[({5-[4-(cyclopropyloxy)phenyl]pyridin-3-yl}amino)methanediyl]bis(phosphonic 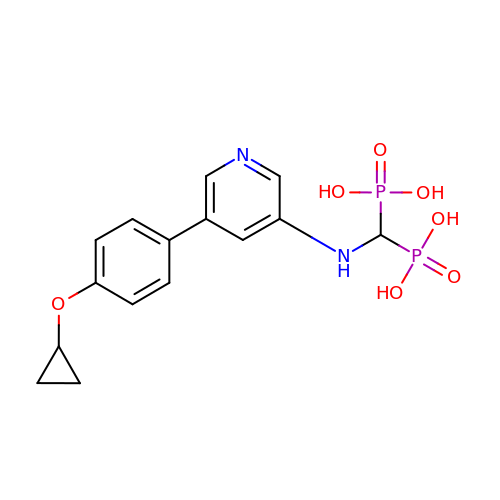acid) | C15 H18 N2 O7 P2 | QCLQOQRSHDMFKS-UHFFFAOYSA-N> MKYLFIFCLFVAGVLAKHEIYDGHAVYQVDVASMDQVKLVHDFENDLMLDVWSDAVPGRPGKVLVPKFKREIFENFLKQSGVQYKLEVENVKEQLELEDQLLAAAAAKSNSTRSRLSFDKIHSYEEVDAYLQELAKEFPNVVTVVEGGKSFEGRSIKYLRISTTNFQDASKPVVMMQSLLHCREWVTLPATLYAIHKLVIDVTESDLINNIDWIILPVANPDGYVHTFGGDRYWRKNRATGYMAGNLCMGVDLNRNFGMNWGTASSSSVCSDTFHGRSAFSEPESSVIRDIIAEHRNRMALYLDIHSFGSMILYGYGNG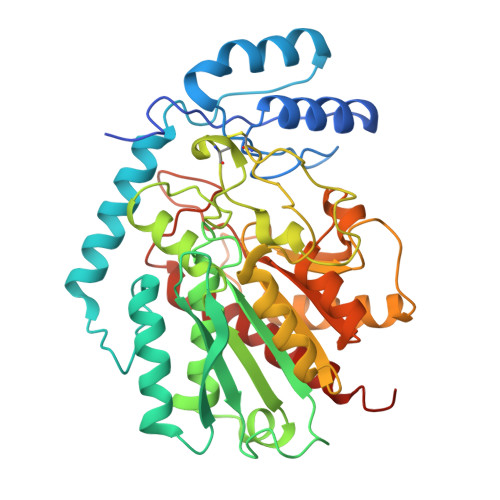VLPSNALQLHLIGVQMAQAIDRVKWSSNKDYIVGNIFHVLYAASGGASDYAMQAAAPFSYTYELPAYRNSVWFDGFLVDPDFIEQAGFETWEGIKVGARAAAAAAKELKKLNTA>GAMGSVHQDSNTGKPISDEKLHLISGKISNKKLPIINSNHDVTWIKTKAMTILGEDGKEIPEFKNKFGYSYIISPVKMDGKYSYYASLLILFETTKNGDDEYEIEDVKFVTAGSTLELKNSLLAVENSQEEGYVTAYPFGILMSDEIKNAFKLTYKNGHWNYMLADLTVKNKLTQETKIYKISLNSKLIIEFLKEVLKENSILK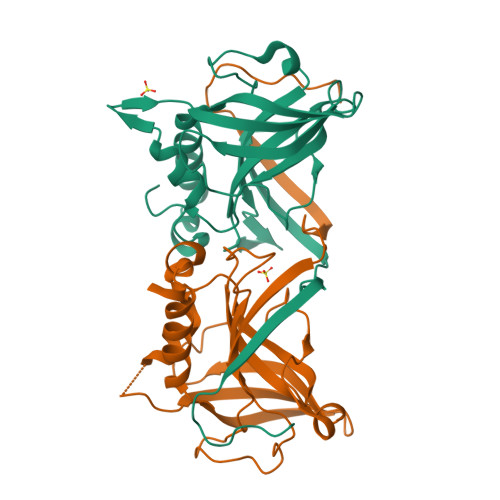DIAGDLFEDI[4x]>GUGCACAC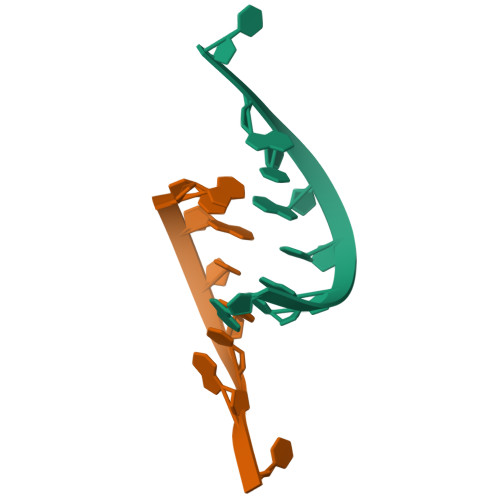[2x]>[4x]MRPLVIILMGSSSDMGHAEKIASELKTFGIEYAIRIGDAHKTAEHVVSMLKEYEALDR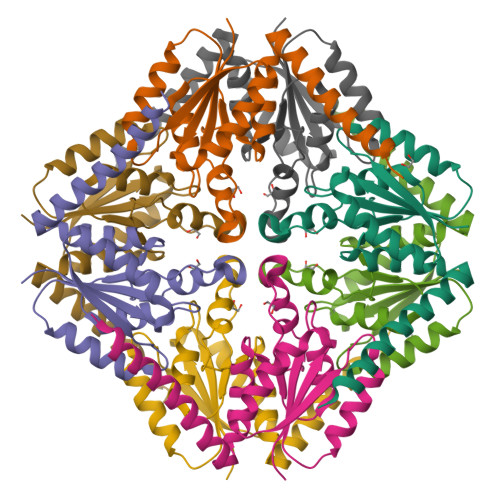PKLYITIAGRSNALSGFVDGFVKGATIACPPPSDSFAGADIYSSLRMPSGISPALVLEPKNAALLAARIFSLYDKEIADSVKSYMESNAQKIIEDDSKLKR> GGFYEIEAIRRKRVRKGKVQYLIKWRGWP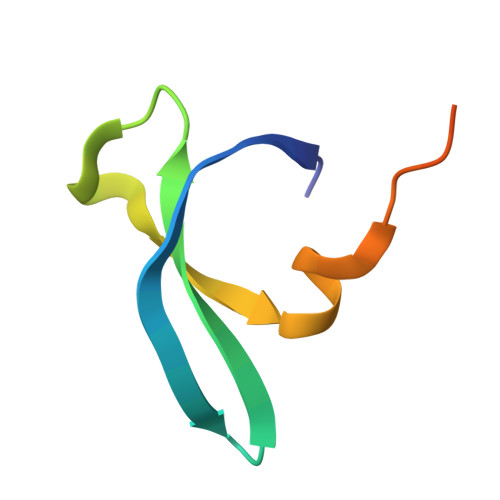ETANTWEPLENLQSIADVIDAFEGSLK> PKALIVYGSTTGNTEYTAETIARELADAGYEVDSRDAASVEAGGLFEGFDLVLLGCSTWNDDSIELQDDFIPLFDSLEETGAQGRKVACFGCGDSSYEYFCGAVDAIEEKLKNLGAEIVQDGLRIDGDPRAARDDIVGWAHDV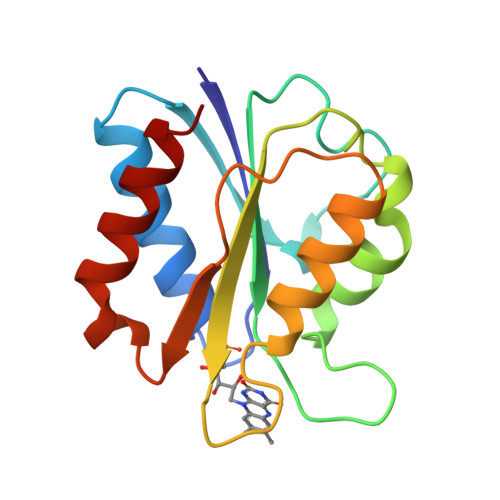RGAI> SNASEGYAGSNTLTIYNWGDYIDPSLITKFEKETGIKVIYQTFDSNEAMMTKIEQGGTTFDIAVPSDYAISKMKEENLLIPLDHSKLPNEKYLDPRFMDLSFDDDNKYSMPYFWGTLGIIYNKEMFPDKNFDTWNALFDPELKNQILLIDGAREVMGLGLNSLGYSLNDTNKAHLQAARDKLETMTPNVKAIVGDEIKLLMADNEAGVAVTFSGEAAEMLSENEDLEYVIPKDGSNLWFDNMVIPKTAKNVDGAHKFINFMLKPENAAINA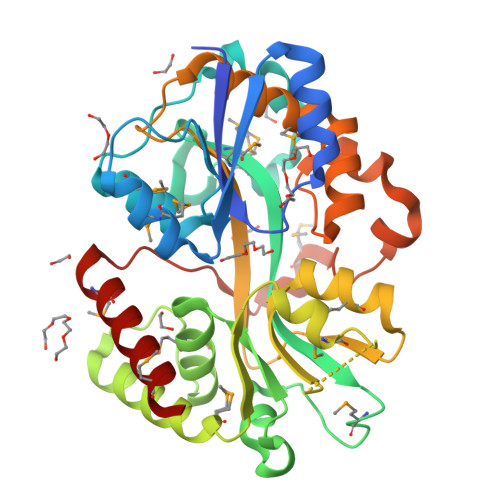EYVGYATPNAKAVELLPKEISSDERFYPDMDELNNLEVYDNLGKRMLSYYNELFLEFKMYRK>[5x]MFPTGWRPKLSESIAASRMLWQPMAAVAVVQIGLLWFSPPVWGQDMVSPPPPIADEPLTVNTGIYLIECYSLDDKAETFKVNAFLSLSWKDRRLAFDPVRSGVRVKTYEPEAIWIPEIRFVNVENARDADVVDISVSPDGTVQYLERFSARVLSPLDFRRYPFDSQTLHIYLIVRSVDTRNIVLAVDLEKVGKNDDVFLTGWDIESFTAVVKPANFALEDRLESKLDYQLRISRQYFSYIPNIILPMLFILFISWTAFWSTSYEANVTLVVSTLIAHIAFNILVETNLPKTPYMTYTGAIIFMIYLFYFVAVIEVTVQHYLKVESQPARAASITRASRIAFPVVFLLANIILAFLFFGF

GLIC is a bacterial homologue of the pentameric ligand-gated ion channels (pLGICs) that mediate the fast chemical neurotransmission of nerve signalling in eukaryotes. Because the activation and allosteric modulation features are conserved among prokaryotic and eukaryotic pLGICs, GLIC is commonly used as a model to study the allosteric transition and structural pharmacology of pLGICs. Unlike the other pLGICs, GLIC displays a particular activation mechanism in which protons, rather than a sizable agonist, trigger ion-channel opening. Here, experimental evidence for carboxylate binding to GLIC is provided by solving its X-ray structures with a series of monocarboxylate and dicarboxylate derivatives, and two carboxylate-binding sites are described: (i) the ‘intersubunit’ site that partially overlaps the canonical pLGIC orthosteric site and (ii) the ‘intrasubunit’ vestibular site, which is only occupied by a subset of the described derivatives.

In attempt to check whether other dicarboxylic acids with different lengths are also able to bind GLIC, we solved crystal structures of GLIC in complex with malonate (diC3) and glutarate (diC5) at 2.9 and 2.65 Å resolution, respectively. The first carboxylic groups of malonate and glutarate occupied the position of acetate, with a similar interaction pattern with Arg77, Glu181 and Arg105. Indeed, all of the monocarboxylic and dicarboxylic acids were found to bind in this pocket with a similar binding mode for the first carboxylic group involving Arg77 and Glu181 from one subunit and Arg105 from the neighbouring sububnit. For dicarboxylates, except for malonate, Asn152 from the complementary subunit contributes to the coordination of the second carboxylic group. For malonate, the molecule is too short to reach the Asn152 side chain and the second carboxylate is thus coordinated by Arg105.> GGCUUAUCAAGAGAGGGGGAGUGACUGGCGCGAAGACCCCCGGCAACCAGAAAUGGUGCCAAUUCCUGCAGCGGAAACGUUGAAAGAUGAGCCG

One especially common junction element is the kink-turn (k-turn). k-turns are elements in double-stranded RNA that introduce a tight kink into the helical axis, with an included angle close to 50°. A standard k-turn comprises a three-nucleotide bulge followed by successive G•A and A•G trans G(sugar edge)•A(Hoogsteen edge) basepairs. k-turns are commonly-occurring motifs that introduce sharp kinks into duplex RNA, thereby facilitating tertiary contacts. Both the folding and conformation of k-turns are determined by their local sequence. k-turns fall into two conformational classes, called N3 and N1, that differ in the pattern of hydrogen bonding in the core. We show here that this is determined by the basepair adjacent to the critical G•A pairs.

We therefore decided to extend the study with a systematic structural analysis of HmKt-7 as a function of the 3b,3n sequence. This was performed in the constant environment of the SAM-I riboswitch, modified by replacing its natural k-turn by HmKt-7 with different 3b,3n sequences. In this way we could observe the effect of changing the 3b,3n sequence alone in an otherwise completely unchanged RNA molecule. Additionally, we hoped we might expand the range of 3b,3n sequences beyond the eight found in the natural k-turns to date. Six are completely new, i.e. 3b,3n = C•A, C–G, C•U, G•G, U–A and U•C, five of which adopt the N1 conformation. The main rules for the ion dependence of folding are that k-turns in which 3b = C (row 2) and 3n = G (column 3) fold in metal ions, 3b,3n = Watson–Crick basepair (ascending diagonal) are not folded by ions and that the latter dominates because 3b,3n = C–G is not folded in metal ions alone. Altogether seven of the new structures are in the N1 conformation, and clearly simply changing the 3b,3n sequence alone is sufficient to induce the structure of Kt-7 to change within the riboswitch environment. Evidently the 3b,3n sequence is the major determinant of the k-turn conformation.>TPLEEAIKDVDVSGVLRYRYDTGNFDKNFLNNSNLNNSKQDHKYRAQVNFSAAIADNFKAFVQFDYNAVDGGTGVDNATNAEKGLFVRQLYLTYTNEDVATSVIAGKQQLNIIWTDNGVDGLVGTGVKVVNNSIDGLTLAAFAVDSFMAAEQGSDLLGQSTYVGNGKNNNDSFKLDSIGNLYGAAAVGSYDLAGGQFNPQLWLAYWDQVAFFYAVDAAYSTTIFDGINWTLEGAYLGNSLDSELDDKKTYANGNLFALKGSIEVNGWDASLGGLYYGDKEKASTVVIEDQGNLGSLLAGEEIFYTTGSRLNGDTGRNIFGYVTGGYTFNETVRVGADFVYGGTKTEATTHLGGGKKLEAVARVDYKYSPKLNFSAFYSYVNLDQGVN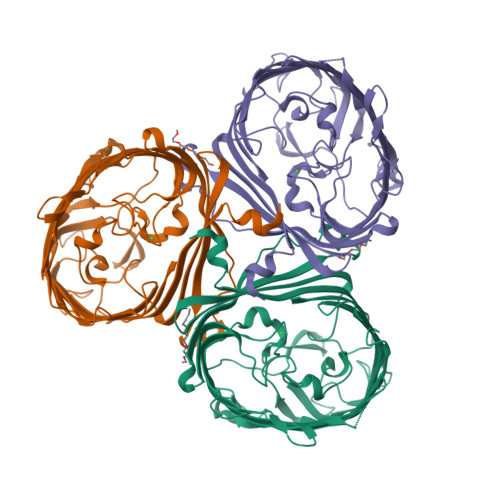TNESADHSTVRLQALYKF[3x]>VSFSVPGLVVEDMSNSRWPAQINGLVVRGNEAQVVHFQNGRCTTEGTLLGTTTLSINSICGLRGLSVSQASVRGAPALTEEMPPLEDEVADGAAATYTLARAADTTLWLRVEEPDGRPYDIFGDQPAPLGTPDFTAVIVGTAIRPRTASGAYLHDAYVDTTPGDADFTPSTGNTKIVLRGGGSGHVGQGHYWQFRPIAVEGGGSRPQYQEYNLPDYAGPTASNHDLAPPVAPRMPGELLLLFESDMPVWDNGAGAAPAQKIHCLLPNEFIT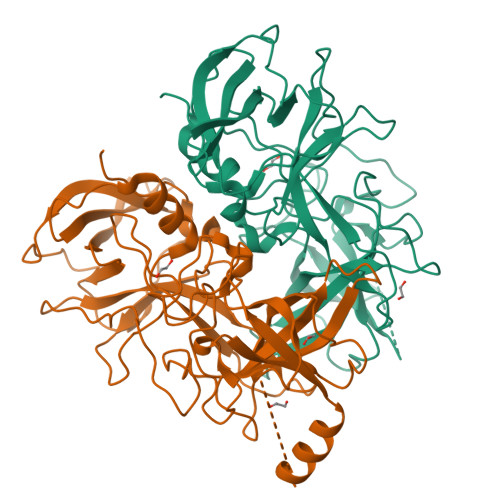HLFDLQAPALAEAALLRYVHPDSGRTLFECKLYREGYMVVAAPAGRLNFPLDGYFRFDSWVSAFYILSPV[2x]Methionine sulfoxide reductases (Msrs) are ubiquitous and highly conserved enzymes that catalyze the reduction of methionine sulfoxide to methionine. MsrA is specific for the S-isomer of methionine sulfoxide and MsrB for the R-isomer. The anaerobic gram-positive bacterium Clostridium oremlandii contains a selenocysteine (Sec)-containing MsrA (CoMsrA). We recently determined the crystal structures of CoMsrA using the Cys version proteins. This enzyme is found to be a structurally unusual MsrA composed of two domains, a catalytic domain and a distinct helical domain absent from other known MsrA structures.

The crystal structure of the ΔH-domain form comprising residues 1–144, corresponding to the catalytic domain, was determined at a resolution of 1.76 Å. In an asymmetric unit, there are two molecules of ΔH-domain protein, but each molecule shows different crystal structures. The final refined model contains chain A comprising 134 residues (7–140) and chain B comprising 137 residues (6–142). The monomer structure of the ΔH-domain protein folds into a similar rolled mixed β-sheet with three helices located at the exterior sides. The dimers are made by swapping of the N-terminus between two molecules. Each N-terminus including residues 6–18 extends outwards from the original molecule of full-length form, intruding between β2 and β3 of another symmetric molecule and forming a complete rolled mixed β-sheet. The ΔH-domain protein predominantly existed as a dimer in solution, which is in agreement with the crystallographic data. In contrast, in dimer B, Cys16 residues are closely located at a distance of 3.6 Å, but no disulfide bond is observed. The C-terminal region, including Tyr140, of the ΔH-domain protein is transformed into a flexible loop from the original helices structure. Loss of interactions with the catalytic domain by deleting the helical domain leads to collapse of the active site, thereby causing a loss of activity.

>[2x]MDTNQKLSIAVFALGCFWGPDAQFGSIKGVVSTRVGYAGGTTNNPSYYNLGDHSESIEIQYDANVITYGELLNIFWNLHNPVYETTNRQYMSRIFYLDDGQKSEALEMKRQIEAANGEKIYTEIVPLENFYLAEGYHQKYYLQN>[4x]MGPVWRKHYITYRINNYTPDMNREDVDYAIRKAFQVWSNVTPLKFSKINTGMADILVVFARGAHGDDHAFDGKGGILAHAF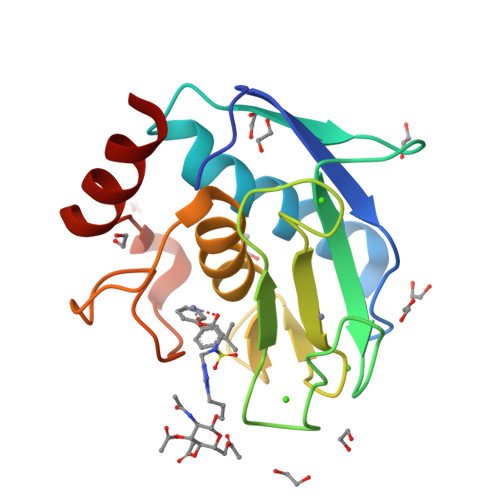GPGSGIGGDAHFDEDEFWTTHSGGTNLFLTAVHQIGHSLGLGHSSDPKAVMFPTYKYVDINTFRLSADDIRGIQSLYG> SIDSALNWDGEMTVTRFDAMTGAHFVIRLDSTQLGPAAGGTRAAQYSNLADALTDAGKLAGAMTLKMAVSNLPMGGGKSVIALPAPRHSIDPSTWARILRIHAENIDKLSGNYWTGPDV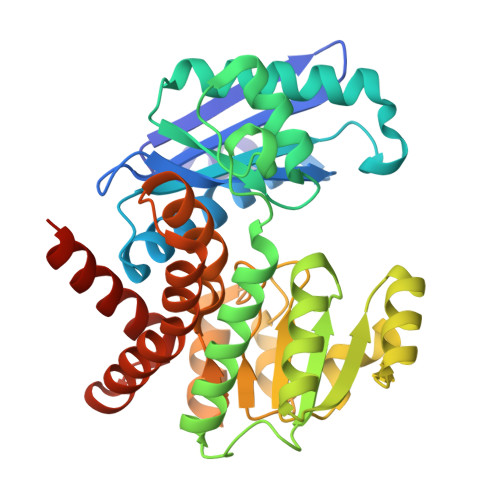NTNSADMDTLNDTTEFVFGRSLERGGAGSSAFTTAVGVFEAMKATVAHRGLGSLDGLTVLVQGLGAVGGSLASLAAEAGAQLLVADTDTERVAHAVALGHTAVALEDVLSTPCDVFAPCAMGGVITTEVARTLDCSVVAGAANNVIADEAASDILHARGILYAPDFVANAGGAIHLVGREVLGWSESVVHERAVAIGDTLNQVFEISDNDGVTPDEAARTLAGRRAREASTTTATA>MTAQYQVQDGVAVITLDNPPVNGLGHSTRLGIVEGMTRALDDAAVKAIVITGAGKAFSGGADIREFNTPKAMQEPTLHSVIRVLEGSSKPVVAAVHSVAMGGGLELALGCNYRVASKGAQIALPEVKLGLLPGAGGTQRLPRVIGLEAAANMIVSGTPVLSEKFAGTKLFDEIVDGDVLPAAVKFAQNVGAATGPHPKVRDLKVRHENPEGYLGFARNTVAAMAKNFPAPLKCLEAVAGSLKPFEQGLKQEREGFLYLVTTPESRALRHAFFGERAASKIPDVPEGTPTRKIEKVAVIGAGTMGGGISMNFLNAGIPVTILETKQEALDRGVGIIRKNYENSAKKGKLTQEKVEQRMGLLSTTLSYDDLKDADLIIEAVFEEMGVKETVFKKLDEVAKQGAILASNTSTLDVNKIASFTKRPQDVVGMHFFSPANVMKLLEVVRGEKTGKDVLATVMQVGKKIKKTAVVSGVCDGFIGNRMIEQYSRQAGYLLDEGALPEQVDKAIEKFGFAMGPFRMGDLAGNDIGWAIRKRRAVDKPEIQYSKTADLLCEMGRFGQKTGAGWYDYKAGDRKPYPNQQVNDMIVQHSKDLGITRRKISDEEIVERLVFALVNEGARILEEGIASKASDIDMVYLTGYGFPLFRGGPMLYADQVGLYNVALSMKRYAKGYHGE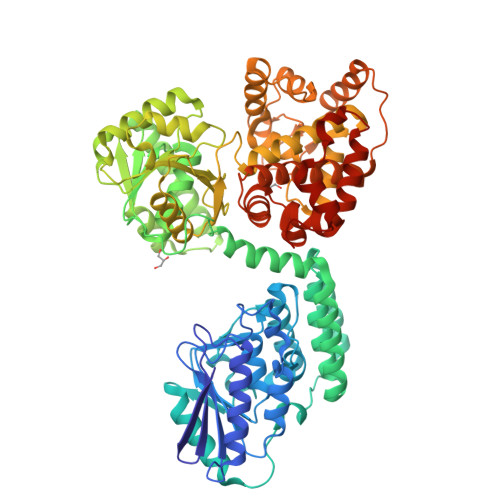AWQVAPLLQKLADEGKGFNGLEHHHHHH[2x]> TITKEGMLHYKAGTSYLGKEHWKTCFVVLSNGILYQY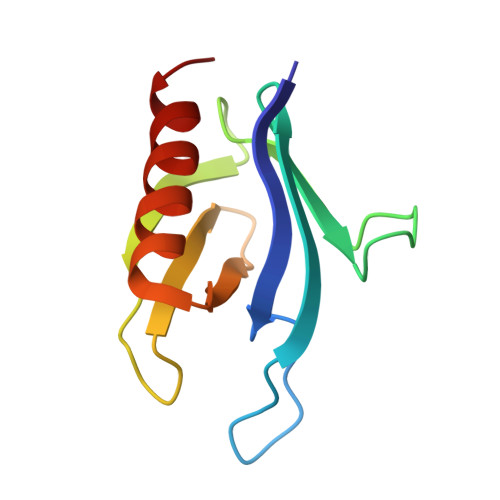PDRTDVIPLLSVNMGGEQCGGCRRANTTDRPHAFQVILSDRPCLELSAESEAEMAEWMQHLCQAVSKG>MEKYTIKETILTFNNEFNDPLDKYYKILSNPKIDTIEFGEKFNQEIDHLIPSNIKVIKFGWTSEFNKDVNFLTESLTEIYYGIYKNHSLEELQNLPKSLLKLKLGDVFNQEIVENVLPGGLTHLTFGEEFNQKIVENVLPGGLTHLTFGEEFNQKIVENVLPNSLTHLSFGDCFNQKITENVLPNSLTYLEFGRNFNQKITENVLPNSLTHLTFGWYFNQQITENVLPNSLTYLEFGRNFNQQITENVLPNSLTYLEFGRNFNQQITENVLPNSLTHITFGNNFNQIITENVLPNSLTHLTFGNNFNQIITENVLPNSLTHLTFGDDFNQIITENVLPNSLTHLTFGDDFNQIITENVLPNSLTHLTFGDDFNQIITENVLPNSLVHLSFGCEFNQEIAEKVLPNSLTYLELGHNFNQKIIENVLPNGLVHLSFGCKFNQEIVENVLPDSLTHLSFGHCFNQKITENVLPNSLTYLELGHNFNQKIIENVLPDRLTYLELGHDFNQKIMENVLPNSLTHLIFGTSFNQNLTENVLPNSLTHLTFGTCFNQKIIENVLPNSLTHLEFG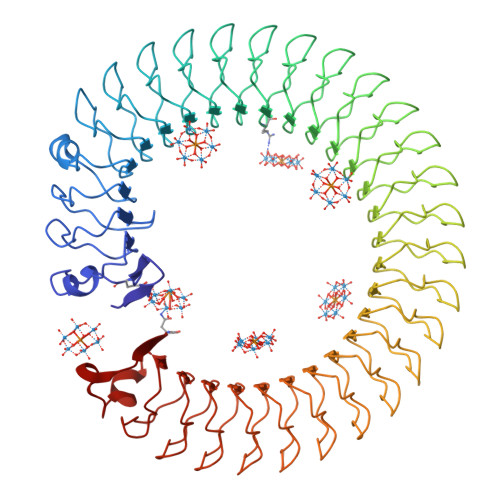PKFNQKITENVLPNSLTHLTFGTSFNQKITENVLPNGLTYLTFGLRFNQKITENVLPCSLTHLTFGWYFNQELTENVLPDTLKVLKIYYGNKDIILKNIDTSKIKFKIEYFNKN[2x]(R)-4-(((S)-1-(((S)-1-amino-4-carboxy-1-oxobutan-2-yl)amino)-4-carboxy-1-oxobutan-2-yl)amino)-3-((3-(3'-chloro-[1,1'-biphenyl]-4-yl)isoxazol-5-yl)methyl)-4-oxobutanoate 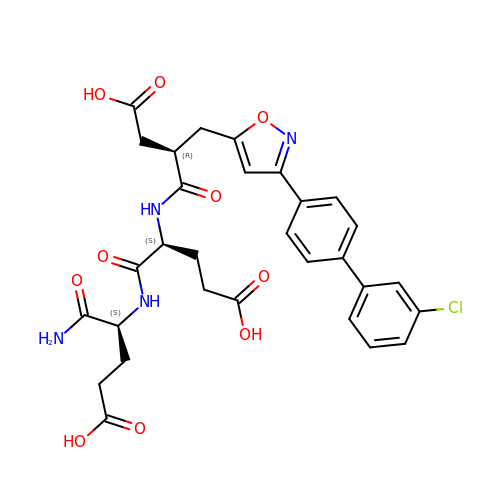| C30 H31 Cl N4 O10 | IXVAVGNSYYZTEW-OIBXWCBGSA-N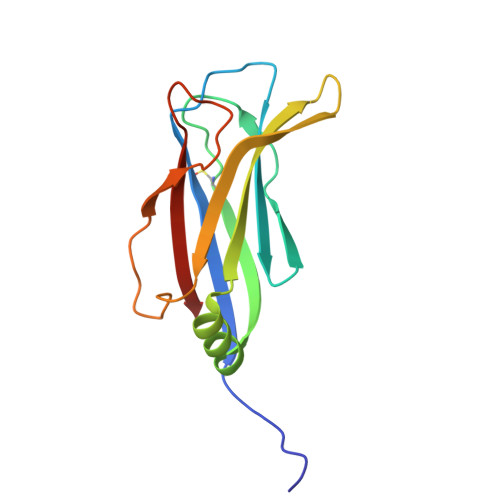> GPHMASKSEQLLIVVSILEGRQFPRSPRLSLVVEARFDGETLSTDPVEHKEQPQFCTELAWELDRRTLHQHRLQRTPIKLQCYAVDSSTSARESVGYIVLDLRSVQEIKQAPKWHPLLSSKYTKLKPALLIGMILENDN4-IODO-3-NITROPHENYL ACETYL-LEUCINYL-LEUCINYL-LEUCINYL-VINYLSULFONE | C28 H43 I N4 O8 S | 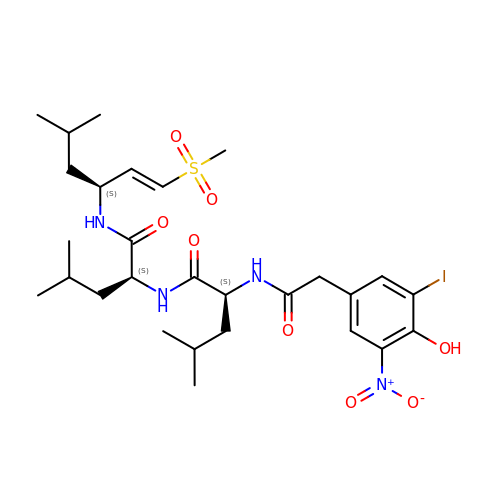RSYTXXARKSZDKY-PUHATCMVSA-N> GSMLEVEKAKLFLHKIPNNVPSAALAQVLSGKFTLDVKQAKTQGRYYCAFALFHSSEDADQAFEHIDGIEMTDSLGLPQKVVIIKLSSGSRASIYVRKMVQDE

In this study, we solved the structure of SDN1, an exonuclease that initiates miRNA degradation by trimming their 3′ ends to generate unmethylated miRNAs that can be further turned over. Arabidopsis SDN1 and SDN2 belong to the DEDD 3′→5′ exonuclease superfamily, characterized by an active core consisting of three separate sequence motifs with four invariant acidic amino acids (DEDD). The Arabidopsis SDN family belongs to the DEDDh subfamily. Our structural and biochemical studies revealed the structural features of SDN1 in substrate recognition and provided insights on how SDN1 uses its DEDDh catalytic domain and the RRM domain cooperatively to degrade free small RNAs and trim miRNAs in miRNA/target RNA duplexes or miRNAs bound by AGO1.

To better understand its structure and function, we conducted crystallographic studies and obtained crystals of the SDN1 CTD (residues 309–409) with mutations in three glutamic acid residues (E329A/E330A/E332A). In the CTD structure, residues 315–409 adopts a βαββαβββ RNA Recognition Motif (RRM) fold, but the N-terminal first α helix (residues 309–314) belongs to the linker connecting the DEDDh and RRM domains. In the SDN1 RRM structure, the six-stranded, antiparallel β sheet forms a positively charged surface and packs against two α-helices. Sequence similarities between SDN1 RRM and other RRM proteins are very low, but two aromatic amino acids that are usually crucial for RNA binding in RRM family members are present in SDN1 RRM (Phe318 in β1 and Phe356 in β3). Mapping all these residues onto the RRM surface reveals that they are mainly located on the antiparallel β sheet (β1, β3, β4, β5, and β6), which is positively charged. Interestingly, NMR titration showed that Phe318 on β1 of SDN1 RRM interacts with RNA, but no large change in chemical shift was observed for Phe356, suggesting that Phe356 may not be involved in RNA binding. Another feature of SDN1 RRM is that its extended β4 and β5 participate in RNA binding (residues Thr378, Asp379, Gly382, and Gln385 detected via NMR titration), whereas most canonical RRMs consist of very short or no β4 and β5. Unlike many RRMs, which exhibit strong substrate binding affinities (in the nM range) and sequence specificities, SDN1 RRM binds RNA weakly in a sequence independent mode. Moreover, canonical RRMs usually fold into a βαββαβ topology, while our structural and NMR titration studies show that SDN1 RRM is composed of a six-stranded antiparallel β sheet with the unconventional extension of β4 and β5, and the two extended β strands are involved in RNA binding. Despite its low RNA binding affinity, the RRM domain is critical to the overall RNA binding affinity and processive enzyme activity of SDN1 by working cooperatively with the DEDDh domain—while the DEDDh domain attacks the 3′ end of an ssRNA, the RRM binds the 5′ region of the RNA.>[3x]MRSLNPLSTPQFDSTDETPASYNLAVRRAAPAVVNVYNRGLNTNSHNQLEIRTLG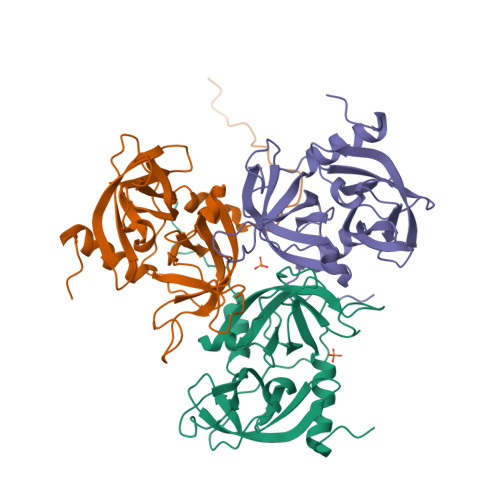SGVIMDQRGYIITNKHVINDADQIIVALQDGRVFEALLVGSDSLTDLAVLKINATGGLPTIPINARRVPHIGDVVLAIGNPYNLGQTITQGIISATGRIGLNPTGRQNFLQTDASINHGNSGGALVNSLGELMGINTLSFDKSNDGETPEGIGFAIPFQLATKIMDKLIRDGRVIRHHHHHH> MDGHNQNQYQNQNQIQQSQQPPLKKYVTQRRSVDVSSPYINLYYNRRHGLPNLVVEPETSYTIDIMPPNAYRGRDRVINLPSKFTHLSSNKVKHVIPAIQWTPEGRRLVVATYSGEFSLWNASSFTFETLMQAHDSAVTTMKYSHDSDWMISGD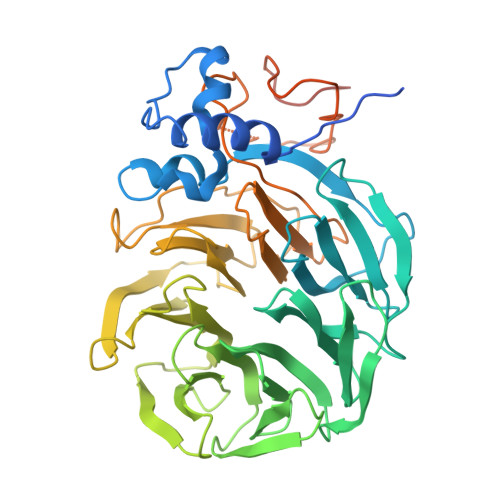ADGMIKIWQPNFSMVKEIDAAHTESIRDMAFSSNDSKFVTCSDDNILKIWNFSNGKQERVLSGHHWDVKSCDWHPEMGLIASASKDNLVKLWDPRSGNCISSILKFKHTVLKTRFQPTKGNLLMAISKDKSCRVFDIRYSMKELMCVRDETDYMTLEWHPINESMFTLACYDGSLKHFDLLQNLNEPILTIPYAHDKCITSLSYNPVGHIFATAAKDRTIRFWTRARPIDPNAYDDPTYNNKKINGWFFGINNDINAVREKSEFGAAPPPPATLEPHALPNMNGFINKKPRQEIPGIDSNIKSSTLPGLSIXXXXX>[3x]PMFIVNTNVPRASVPEGFLSELTQQLAQATGKPAQYIAVHV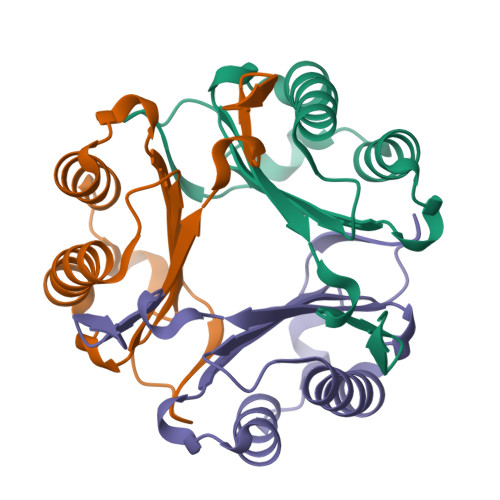VPDQLMTFSGTNDPCALCSLHSIGKIGGAQNRNYSKLLCGLLSDRLHISPDRVYINYYDMNAANVGWNGSTFA>[2x]MDLPEIVASGDPVLHEKAREVDPGEIGSERIQKIIDDMIKVMRLAPGVGLAAPQ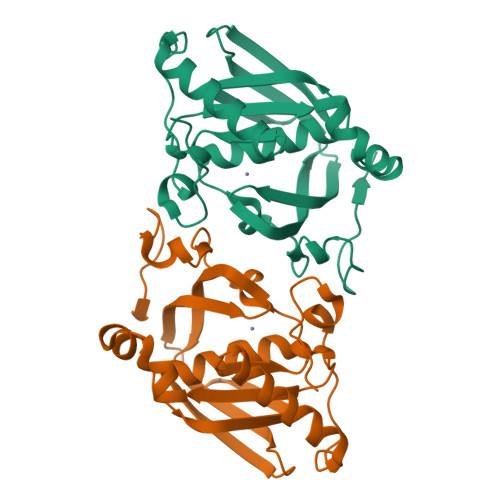IGVPLRIIVLEDTKEYISYAPKEEILAQERRHFDLMVMVNPVLKERSNKKALFFEGCLSVDGFRAAVERYLEVVVTGYDRQGKRIEVNASGWQARILQHECDHLDGNLYVDKMVPRTFRTVDNLDLPLAEGCPKLGSHHHHHH>[2x]MNIYTFDFDEIESQEDFY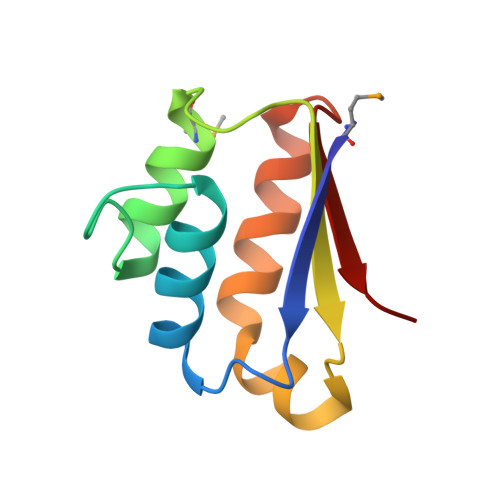RDFSQTFGLAKDKVRDLDSLWDVLMNDVLPLPLEIEFVHLGEKTRRRFGALILLFDEAEEELEGHLRFNVRH> VGLTTLFWLGAIGMLVGTLAFAWAGRDAGSGERRYYVTLVGISGIAAVAYVVMALGVGWVPVAERTVFAPRYIDWILTTPLIVYFLGLLAGLDSREFGIVITLNTVVMLAGFAGAMVPGIERYALFGMGAVAFLGLVYYLVGPMTESASQRSSGIKSLYVRLRNLTVILWAIYPFIWLLGPPGVALLTPTVDVALIVYLDLVTKVGFGFIALDAAATLRAEHGESLAGVDTDAPAVADEN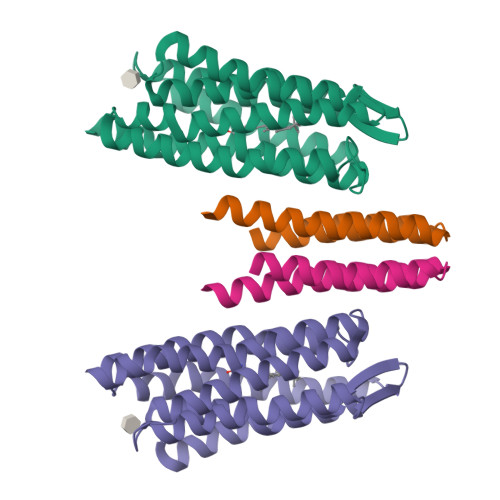SHHHHHHH;> ALNVSRLLLPSRVRHSYTGKMGAVFIFVGALTVLFGAIAYGEVTAAAATGDAAAVQEAAVSAILGLIILLGINLGLVAATLGGDTAASLSTLAAKASRMGDGDLDVELETRRENSHHHHHHH A decade-long search for a protein pair mediating this event in mammals culminated in the identification of the glycosylphosphatidylinositol (GPI)-anchored glycoprotein Juno as the egg plasma membrane receptor of sperm Izumo1 1, 2. The Juno–Izumo1 interaction was shown to be essential for fertilization since mice lacking either gene exhibit sex-specific sterility, making these proteins promising non-hormonal contraceptive targets 1, 3. Here, we report the crystal structure of Juno and find that the overall fold is similar to that of FRα and FRβ but with significant flexibility within the area that corresponds to the rigid ligand-binding site of these bona fide folate receptors. Whereas FR homologues are found in all vertebrate classes, Juno appears restricted to mammals. Together with this observation, our studies suggest that the molecular basis of mammalian gamete recognition evolved from an ancestral FR that lost the ability to bind vitamin B9, but gained the ability to recognize Izumo1.

To gain insights into how Juno recognizes Izumo1, we expressed the complete ectodomain of mouse Juno (residues G20–A221) as a soluble protein in glycosylation-impaired mammalian cells (see Supplemental Experimental Procedures). Following enzymatic trimming of N-glycans, affinity-purified Juno behaved as a monomer by size-exclusion chromatography and yielded a ∼10 μm thick crystal that diffracted to 2.7 Å resolution. Juno consists of nine α-helices and six short β-strands, which adopt the same fold of FRα and FRβ 4, 5 and riboflavin-binding protein (RfBP). The bulk of the structure, including four core α-helices and seven disulfide bonds, can be superimposed onto the ligand-bound form of human FRα and FRβ with root mean square deviations (RMSD) of 1.4 Å and 1.6 Å over 166 and 167 residues, respectively. Although glycosylation at N73 is important for secretion of Juno (lane 1), there is no electron density for the loop carrying the corresponding GlcNAc, suggesting that this conserved carbohydrate affects protein solubility rather than folding. A crystal contact, however, fixes the position of the N-glycan at N185, which is neither conserved nor required for secretion (lane 2). Despite their overall similarity, there are striking local differences between the structure of Juno and that of FRs and RfBP. Whereas in the latter proteins three highly ordered loops generate a deep binding pocket for the respective ligands 4, 5, 6, the corresponding regions of Juno are either largely disordered (loops 1 and 3) or adopt a very different conformation (loop 2). Taken together with sequence alignments, these observations suggest that — in addition to key amino acid substitutions such as D103A 1, 4 — structural disorder or displacement of conserved pocket residues important for ligand recognition in FRα contribute to the inability of Juno to bind vitamin B9.

>[2x]ETGAAAGDKLLSVCMNSKRHKQEPGPEDELYQECRPWEDNACCTRSTSWEAHLEEPLLFNFSMMHCGLLTPACRKHFIQAICFHECSPNLGPWIQPVVPNGQEEQRVWGVPLCQEDCEDWWRACHSSLTCKSNWLHGWDWSEEKKHCPAHEPCLPFSYHFPTPDDLCEKIWNNTFKASPERRNSGRCLQKWFEPTLSNPNVEVALHFAHHHHHHHH>MGSSHHHHHHSQDPMTDSTTHYTRPDVAAFLAFLNAQEGPKMEEMPPAGAREMMRVMGQLADVPRGEIAKVEDRMIPGPDGDIPIRLYDNRPDREAGPVMVFYHGGGWVIGDLETHDPYCAEAARILDMPVIAIDYRLAPEHPFPAAPIDCEAATRWVADNIACTGLVLSGDSAGGNLTIVTALALRDEPAAKPVIAIHPIYPAVTTHNDWQSYRDFGEGHLLTEGSMTWFGNHYAADPADRRAAPIDFPADGLPPTLLITASLDPLRDQGRAYAAKLIEAGVPTTYREAKGTIHGYICLAQGIPSAKDDIRGALTVLKAIVAEATGAA[2x]

Herein, we identified from a library of lipases/esterases/acyltransferases and variants thereof a lipase originating from Sphingomonas sp. HXN-200 (SpL) able to form amides in aqueous solution starting from a broad scope of sterically demanding heteroaromatic ethyl esters as well as aliphatic amines, reaching isolated yields up to 99% on preparative scale and space time yields of up to 864 g L–1 d–1; thus, in selected cases, the amide was formed within minutes. SpL is a hormone-sensitive lipase-like (HSL-like) protein adopting the alpha-beta hydrolase fold, with a helical lid domain over the active site cavity with the catalytic triad. The common Ser-His-Asp catalytic triad was located at positions Ser159, His281, and Asp251. Mutational and structural studies revealed that an aspartate next to the catalytically active serine is highly beneficial for the observed activity, which has not been described before, showing that a catalytic tetrad is actually required (Asp-Ser-His-Asp) for SpL for efficient amide formation in aqueous buffer.

To gain insights into the mechanism of amide formation catalyzed by lipase SpL, its structure was determined by X-ray crystallography. Diffraction data were collected under cryo-conditions from native crystals, as well as from crystals soaked with benzylamine 2a or the amide N-benzyl-2-pyridinecarboxamide 3a,a leading to data sets with resolutions of 2.0, 1.6, and 1.8 Å, respectively. Furthermore, two funnel-shaped channels leading from the surface to the catalytic triad or actually the tetrad were identified. Next to Ser159 of the catalytically active triad, an aspartate (Asp158) caught our attention as it is not present, e.g., in the lipase from C. antarctica B (CalB). The aspartate next to the catalytically active serine may represent an extension of the classical triad Ser-His-Asp/Glu42−44 in the lipase mechanism to a tetrad. Furthermore, the crystal structure showed that the enzyme possesses two access tunnels to the active site, probably one for the ester and one for the amine, another feature not described before. This feature allows for bringing together two sterically demanding substrates, the ester and amine, without interfering with each other.> IVGGSDSREGAWPWVVALYFDDQQVCGASLVSRDWLV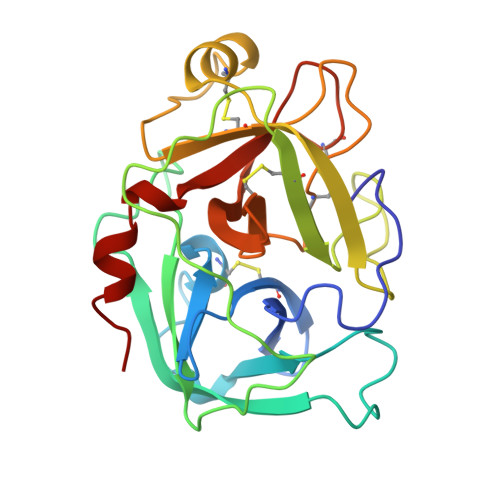SAAHCVYGRNMEPSKWKAVLGLHMASNLTSPQIETRLIDQIVINPHYNKRRKNNDIAMMHLEMKVNYTDYIQPICLPEENQVFPPGRICSIAGWGALIYQGSTADVLQEADVPLLSNEKCQQQMPEYNITENMVCAGYEAGGVDSCQGDSGGPLMCQENNRWLLAGVTSFGYQCALPNRPGVYARVPRFTEWIQSFLH> GRFERIKKPLKSDMNVVPYI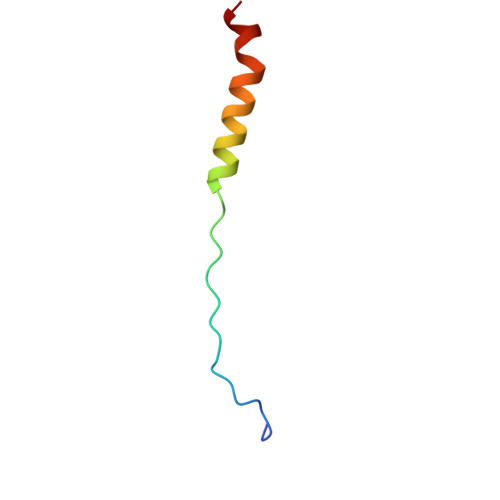DVMLVLLVIFMVTAPMITS> AVNCNEKIVVLLQRLKPEIKDVIEQLNLVTTWLQLQIPRIEDGNNFGVAVQEKVFELMTSLHTKLEGFHTQISKYFSERGDAVTKAAKQPHVGDYRQLVHELDEAEYRDIRLMVMEIRNAYAVLYD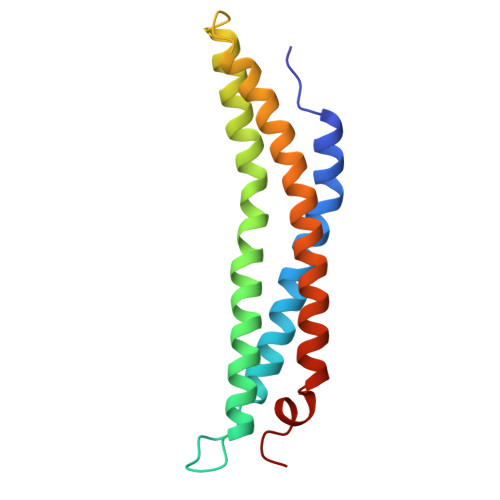IILKNFEKLKKPRG>MASWSHPQFEKGADDDDKVPDPTSAIGVLTSGGDAQGMNAAVRAVVRMGIYVGAKVYFIYEGYQGMVDGGSNIAEADWESVSSILQVGGTIIGSARCQAFRTREGRLKAACNLLQRGITNLCVIGGDGSLTGANLFRKEWSGLLEELARNGQIDKEAVQKYAYLNVVGMVGSIDNDFCGTDMTIGTDSALHRIIEVVDAIMTTAQSHQRTFVLEVMGRHCGYLALVSALACGADWVFLPESPPEEGWEEQMCVKLSENRARKKRLNIIIVAEGAIDTQNKPITSEKIKELVVTQLGYDTRVTILGHVQRGGTPSAFDRILASRMGVEAVIALLEATPDTPACVVSLNGNHAVRLPLMECVQMTQDVQKAMDERRFQDAVRLRGRSFAGNLNTYKRLAIKLPDDQIPKTNCNVAVINVGAPAAGMNAAVRSAVRVGI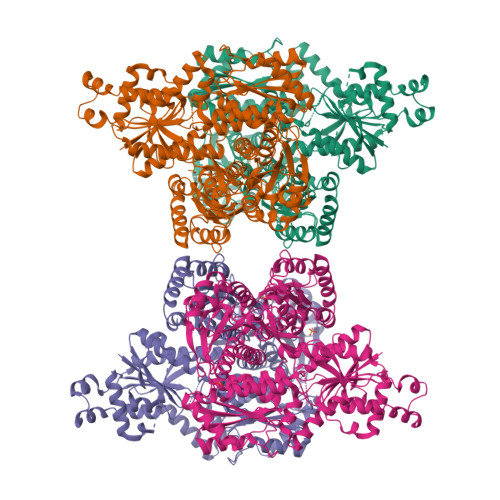ADGHRMLAIYDGFDGFAKGQIKEIGWTDVGGWTGQGGSILGTKRVLPGKYLEEIATQMRTHSINALLIIGGFEAYLGLLELSAAREKHEEFCVPMVMVPATVSNNVPGSDFSIGADTALNTITDTCDRIKQSASGTKRRVFIIETMGGYCGYLANMGGLAAGADAAYIFEEPFDIRDLQSNVEHLTEKMKTTIQRGLVLRNESCSENYTTDFIYQLYSEEGKGVFDCRKNVLGHMQQGGAPSPFDRNFGTKISARAMEWITAKLKEARGRGKKFTTDDSICVLGISKRNVIFQPVAELKKQTDFEHRIPKEQWWLKLRPLMKILA[4x]The Aurora family is a well conserved and well characterized group of serine-threonine kinases involved in the normal progression of mitosis. Mammalian cells possess three Aurora kinase isoforms (Aurora A, B and C) that exhibit different subcellular localizations and have distinct functional roles. The most conserved C-terminal region of INCENP (the so-called IN-box) is sufficient to bind and stimulate the catalytic activity of Aurora B. The CPC complex is involved in numerous mitotic functions, and the timing and mechanisms of each of these events are carefully regulated by its localization within mitosis. As expected, deregulation of Aurora kinases has drastic intra­cellular consequences, rendering these kinases attractive drug targets for small-molecule inhibitor development, targeting the active-site binding pocket which binds the ATP substrate.

Despite the high reported specificity of barasertib towards Aurora B, structural data describing the interaction between barasertib and Aurora B are still lacking. In this context, we sought to investigate this inhibition mechanism at the atomic level. For this purpose, we employed the previously described X. laevis Aurora B–INCENP complex as a structural template. The sequence identity between the catalytic kinase domains of X. laevis and Homo sapiens Aurora B is significantly high. We determined the crystal structure of the X. laevis Aurora B–INCENP complex at 1.5 Å resolution, highlighting the binding of the active form of barasertib to the ATP active site. Here, the first structure of the Xenopus laevis Aurora B–INCENP complex bound to the clinically relevant small molecule barasertib was determined. The binding properties of this inhibitor to the Aurora B active site are analyzed and reported. Of the many Aurora B inhibitors that have been reported in the literature, in recombinant enzyme assays barasertib shows a higher selectivity, with more than a 1000-fold greater potency, for Aurora B than for Aurora A, with IC50 values of 1 nM and 1.4 µM, respectively. Consistent with the inhibition of Aurora B kinase, the addition of barasertib to tumour cells in vitro induces chromosome misalignment, prevents cell division and consequently reduces cell viability and induces apoptosis. During refinement of the Aurora B–INCENP–barasertib structure, we noticed extra electron density corresponding to a well ordered arginine residue, Arg847INCENP, in close proximity to the activation loop (data not shown). The structure of the kinase domain was not perturbed and it adopts a highly similar overall conformation to the previous published structures of the catalytic domain both alone and in complex with small-molecule inhibitors.

>[2x]QNTALAEMPKRKFTIDDFDIGRPLGKGKFGNVYLAREKQNKFIMALKVLFKSQLEKEGVEHQLRREIEIQSHLRHPNILRMYNYFHDRKRIYLMLEFAPRGELYKELQKHGRFDEQRSATFMEELADALHYCHERKVIHRDIKPENLLMGYKGELKIADFGWSVHAPSLRRRTMCGTLDYLPPEMIEGKTHDEKVDLWCAGVLCYEFLVGMPPFDSPSHTETHRRIVNVDLKFPPFLSDGSKDLISKLLRYHPPQRLPLKGVMEHPWVKANSRRVLPPVYQSTQS;>[2x]PIPAWASGNLLTQAIRQQYYKPIDVDRMYGTIDSPKLEELFNKS>[15x]MEQTQKLKLNLQHFASNNVKPQVFNPDNVMMHEKKDGTLMNEFTTPILQEVMENSKIMQLGKYEPMEGTEKKFTFWADKPGAYWVGEGQKIETSKATWVNATMRAFKLGVILPVTKEFLNYTYSQFFEEMKPMIAEAFYKKFDEAGILNQGNNPFGKSIAQSIEKTNKVIKGDFTQDNIIDLEALLEDDELEANAFISKTQNRSLLRKIVDPETKERIYDRNSDSLDGLPVVNLKSSNLKRGELITGDFDKLIYGIPQLIEYKIDETAQLSTVKNEDGTPVNLFEQDMVALRATMHVALHIADDKAFAKLVPADKRTDSVPGEV;>[12x]MLKVNEFETDTDLRGNINYLFNDEANVVYTYDGTESDLLQNVNEVSKYIEHHMDYQRPRLKVLSDYYEGKTKNLVELTRRKEEYMADNRVAHDYASYISDFINGYFLGNPIQYQDDDKDVLEAIEAFNDLNDVESHNRSLGLDLSIYGKAYELMIRNQDDETRLYKSDAMST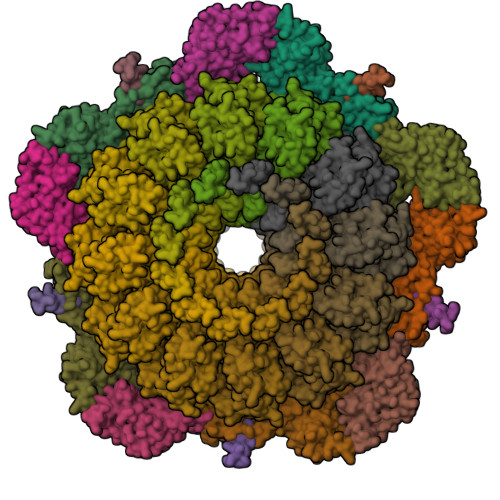FIIYDNTVERNSIAGVRYLRTKPIDKTDEDEVFTVDLFTSHGVYRYLTNRTNGLKLTPRENSFESHSFERMPITEFSNNERRKGDYEKVITLIDLYDNAESDTANYMSDLNDAMLLIKGNLNLDPVEVRKQKEANVLFLEPTVYVDAEGRETEGSVDGGYIYKQYDVQGTEAYKDRLNSDIHMFTNTPNMKDDNFSGTQSGEAMKYKLFGLEQRTKTKEGLFTKGLRRRAKLLETILKNTRSIDANKDFNTVRYVYNRNLPKSLIEELKAYIDSGGKISQTTLMSLFSFFQDPELEVKKIEEDEKESIKKAQKGIYKDPRDINDDEQDDDTKDTVDKKE> GPHMLEREKIYQWINELSSPETRENALLELSKKRESVPDLAPMLWHSFGTIAALLQEIVNIYPSINPPTLTAHQSNRVCNALALLQCVASHPETRSAFLAAHIPLFLYPFLHTVSKTRPFEYLRLTSLGVIGALVKTDEQEVINFLLTTEIIPLCLRIMESGSELSKTVATFILQKIL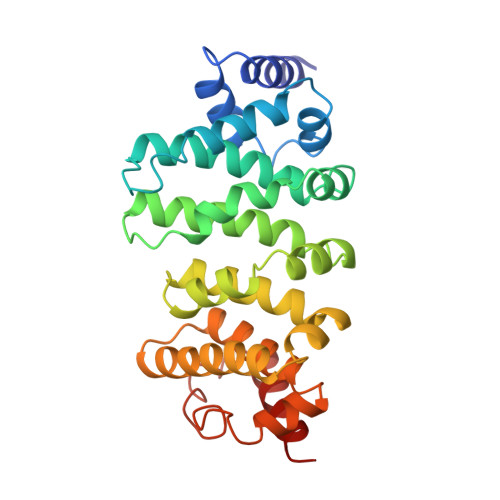LDDTGLAYICQTYERFSHVAMILGKMVLQLSKEPSARLLKHVVRCYLRLSDNPRAREALRQCLPDQLKDTTFAQVLKDDTTTKRWLAQLVKNLQE> GGAVDSTVYKGQVLKSLDRNNPVRQNNDPLPGRIRYRALDYSEVEVPFGDKDQKGDFTLRHGDWVQFLLATDRRDQLQRATSIALLDETFKVSGEKREQGTIASLKEGFGFLRCVERQARLFFHFTEVLDTSREIDINDEV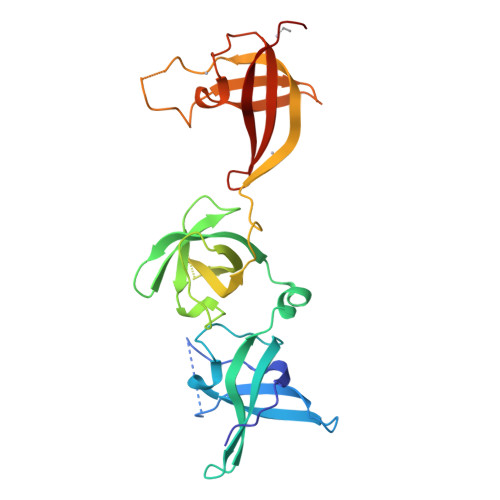EFTVIQEPGLAYNNSRLQAIRIKHLPPNSVQFETLVASNIEGCVTREAPKSPIKSQDRVEGGVITYEHADVKKTIMYFLKDCEKPPRIGERVRFDIYMVKRNKECIAVNVQQVSLH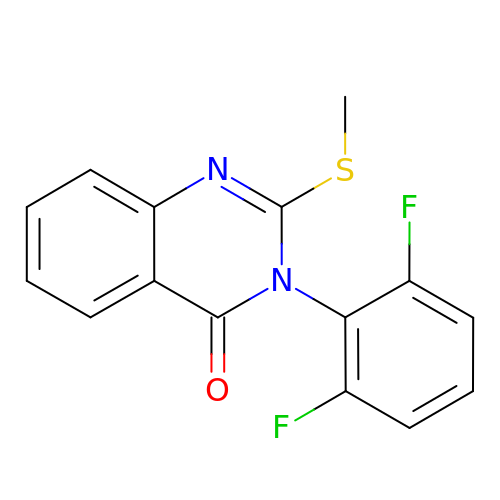3-(2,6-difluorophenyl)-2-(methylthio)quinazolin-4(3H)-one | C15 H10 F2 N2 O S | BFNBJSXMXXQLAW-UHFFFAOYSA-N>[2x]GSRPATPPVTPPSREGHVADLDRFPQDLRVYAMKAGADRQLLPFTEQAAQDARWNRRFFAPWRMTRISVPVKDVAAPFGTDGRPRGYAENLLPWDVTRWGALASGAALDLYPSQAWKGIVVSNSALREVPTLRPMFTAPTRAGQGYPFDMFQRTAVWMGTPVFVGHATADRAWLYVETAFAAGWMPAADVARVDDA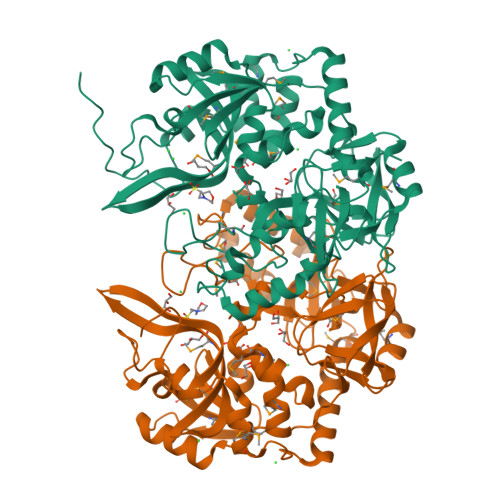FMTRYESGSLAAILRDDTSLNGADGTHLATAHIGTVLPLSGASQVGRTVLVPVRAPEGHAVVVPVLLTSGEAAQKPVPLTPGNMAELGNRMMGQPYGWGGLYEDRDCSSTLRDLFTPFGLWLPRNSASQAKAGRYVDIAKLDADDKEARIVAEGVPFMTLLWLRGHITLYLGLHEGQAAMFHNMWGIRTHRGGVEGRYVLGRAVVTSTRPGLDVPGNDNADGLLGRMQGMSILPGGAQ>EHTHSEREKRVSNAVEFLLDSRVRRTPTSSKVHFLKSKGLSAEEIC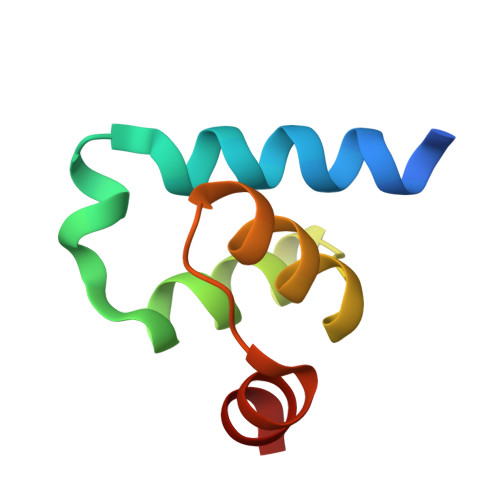EAFTKVGQPKTLNEIKRILS[4x]>MNHKVHHHHHHIEGRHMKAYMFPGQGSQAKGMGRALFDAFPALTARADGVLGYSIRALCQDDPDQRLSQTQFTQPALYVVNAL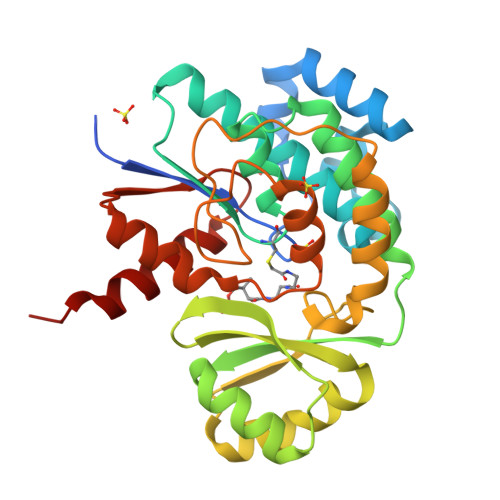SYLKRREEEAPPDFLAGHCLGEFSALFAAGVFDFETGLALVKKRGELMGDARGGGMAAVIGLDEERVRELLDQNGATAVDIANLNSPSQVVISGAKDEIARLQVPFEAAGAKKYTVLRVSAAFHSRFMRPAMVEFGRFLEGYDFAPPKIPVISNVTARPCKADGIRAALSEQIASPVRWCESIRYLMGRGVEEFVECGHGIVLTGLYAQIRRDAQPLVV[2x];>[2x]GSHMPAGAGQDGRRIARIEEDLRRLVSARIEAPSQAVDAEESFFSLGVDSVALQEITETLERTYGSLPPTLLFENPNIRQLARYLAERVPARSA> MYWVRRKTIGGSGLPYTENEILEWRKEGVKRVLVLPEDWE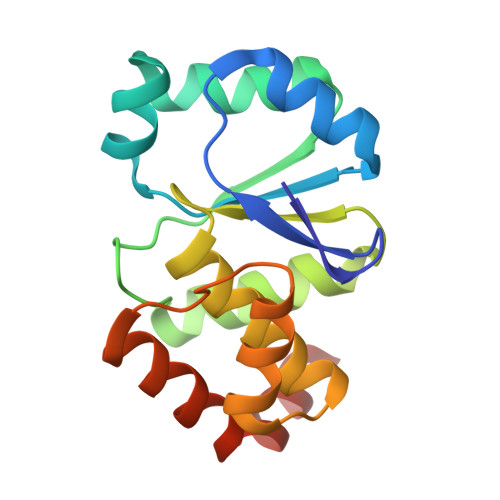IEESWGDKDYYLSILKKNGLQPLHIPIPDGGVPSDSQFLTIMKWLLSEKEGNLVHSVGGIGRTGTILASYLILTEGLEVESAIDEVRLVRPGAVQTYEQEMFLLRVEGMRKSWLKNIYSNS>MSRRAPMFKPLPITLQRGALRLEPLVEADIPELVSLAEANREALQYMDGPTRPDWYRQSLAEQREGRALPLAVRLGVQLVGTTRFAEFLPALPACEIGWTWLDQAQHGSGLNRMIKYLMLKHAFDNLRMVRVQLSTAASNLRA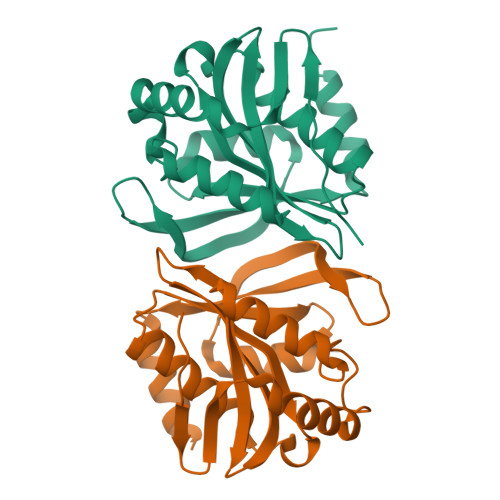QGAIDKLGAQREGVLRNHRRLAGGRLDDTFVYSITDHEWPQVKAALEASFTG[4x]> MITTPLVHVASVEKGRSYEDFQKVYNAIALKLREDDEYDNYIGYGPVLVRLAWHISGTWDKHDNTGGSYGGTYRFKKEFNDPSNAGLQNGFKFLEPIHKEFPWISSGDLFSLGGVTAVQEMQGPKIPWRCGRVDTPEDTTPDNGRLPDADKDAGYVRTFFQRLNMNDREVVALMGAHALGKTHLKNSGYEGPWGAANNVFTNEFYLNLLNEDWKLEKNDANNEQWDSKSGYIMLPTDYSLIQDPKYLSIVKEYANDQDKFFKDFSKAFEKLLENGITF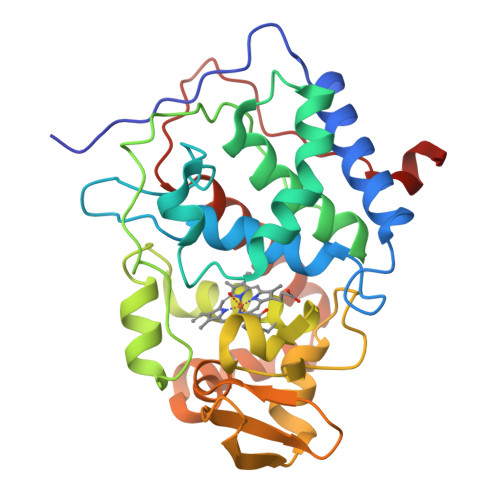PKDAPSPFIFKTLEEQGL> PKTEVSVSAFALLFSEMVQYCQSRVYSVSELQARLADMGQGVGASLLDVLVMREKN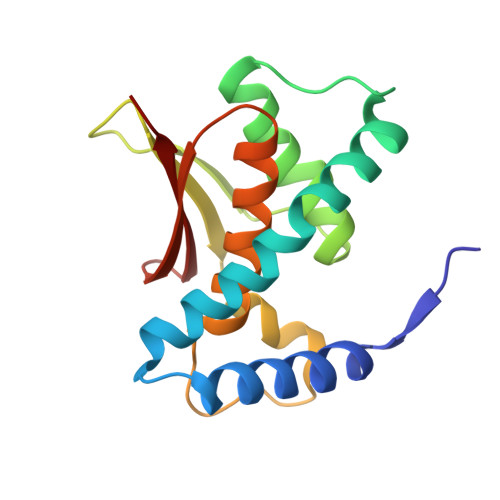GKRETKVLNILLFIKVNVWKALFGKEADKLEQANDDDKTYYIIEKEPLINAYISVPKENSTLNCAAFTGGIVEAILTHSGFPAKVTVHWHKGTTLMIKFDE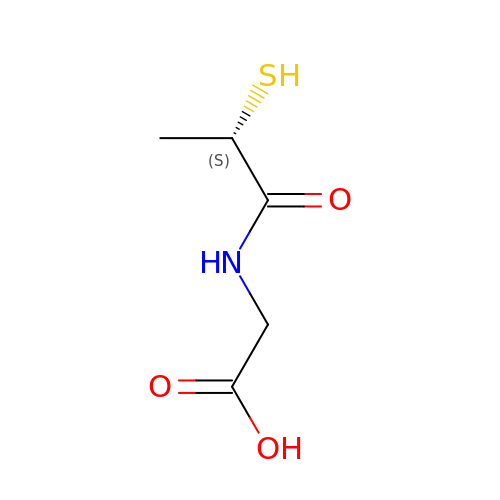TIOPRONIN | C5 H9 N O3 S | YTGJWQPHMWSCST-VKHMYHEASA-N> MLGTGPAAATTAATTSSNVSVLQQFASGLKSRNEETRAKAAKELQHYVTMELREMSQEESTRFYDQLNHHIFELVSSSDANERKGGILAIASLIGVEGGNATRIGRFANYLRNLLPSNDPVVMEMASKAIGRLAMAGDTFTAEYVEFEVKRALEWLGADRNEGRRHAAVLVLRELAISVPTFFFQQVQPFFDNIFVAVWDPKQAIREGAVAALRACLILTTQREPKEMQKPQWYRHTFEEAEKGFDETLAKEKGMNRDDRIHGALLILNELVRISSMEGERLREEMEEITQQQLVHDKYCKDLMGFGTKPRHITPFTSFQAVQPQQSNALVGLLGYSSHQGLMGFGTSPSPAKSTLVESRCCRDLMEEKFDQVCQWVLKCRNSKNSLIQMTILNLLPRLAAFRPSAFTDTQYLQDTMNHVLSCVKKEKERTAAFQALGLLSVAVRSEFKVYLPRVLDIIRAALPPKDFAHKRQKAMQVDATVFTCISMLARAMGPGIQQDIKELLEPMLAVGLSPALTAVLYDLSRQIPQLKKDIQDGLLKMLSLVLMHKPLRHPGMPKGLAHQLASPGLTTLPEASDVGSITLALRTLGSFEFEGHSLTQFVRHCADHFLNSEHKEIRMEAARTCSRLLTPSIHLISGHAHVVSQTAVQVVADVLSKLLVVGITDPDPDIRYCVLASLDERFDAHLAQAENLQALFVALNDQVFEIRELAICTVGRLSSMNPAFVMPFLRKMLIQILTELEHSGIGRIKEQSARMLGHLVSNAPRLIRPYMEPILKALILKLKDPDPDPNPGVINNVLATIGELAQVSGLEMRKWVDELFIIIMDMLQDSSLLAKRQVALWTLGQLVASTGYVVEPYRKYPTLLEVLLNFLKTEQNQGTRREAIRVLGLLGALDPYKHKVNIGMIDQSRDASAVSLSESKSS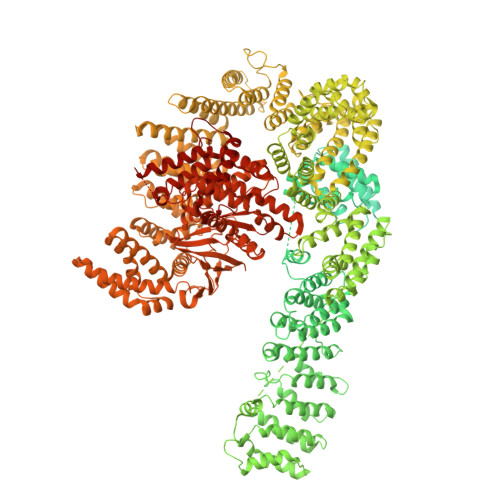QDSSDYSTSEMLVNMGNLPLDEFYPAVSMVALMRIFRDQSLSHHHTMVVQAITFIFKSLGLKCVQFLPQVMPTFLNVIRVCDGAIREFLFQQLGMLVSFVKSHIRPYMDEIVTLMREFWVMNTSIQSTIILLIEQIVVALGGEFKLYLPQLIPHMLRVFMHDNSPGRIVSIKLLAAIQLFGANLDDYLHLLLPPIVKLFDAPEAPLPSRKAALETVDRLTESLDFTDYASRIIHPIVRTLDQSPELRSTAMDTLSSLVFQLGKKYQIFIPMVNKVLVRHRINHQRYDVLICRIVKGYTLADEEEDPLIYQHRMLRSGQGDALASGPVETGPMKKLHVSTINLQKAWGAARRVSKDDWLEWLRRLSLELLKDSSSPSLRSCWALAQAYNPMARDLFNAAFVSCWSELNEDQQDELIRSIELALTSQDIAEVTQTLLNLAEFMEHSDKGPLPLRDDNGIVLLGERAAKCRAYAKALHYKELEFQKGPTPAILESLISINNKLQQPEAAAGVLEYAMKHFGELEIQATWYEKLHEWEDALVAYDKKMDTNKDDPELMLGRMRCLEALGEWGQLHQQCCEKWTLVNDETQAKMARMAAAAAWGLGQWDSMEEYTCMIPRDTHDGAFYRAVLALHQDLFSLAQQCIDKARDLLDAELTAMAGESYSRAYGAMVSCHMLSELEEVIQYKLVPERREIIRQIWWERLQGCQRIVEDWQKILMVRSLVVSPHEDMRTWLKYASLCGKSGRLALAHKTLVLLLGVDPSRQLDHPLPTVHPQVTYAYMKNMWKSARKIDAFQHMQHFVQTMQQQAQHAIATEDQQHKQELHKLMARCFLKLGEWQLNLQGINESTIPKVLQYYSAATEHDRSWYKAWHAWAVMNFEAVLHYKHQNQARDEKKKLRHASGANITNATTAATTAATATTTASTEGSNSESEAESTENSPTPSPLQKKVTEDLSKTLLMYTVPAVQGFFRSISLSRGNNLQDTLRVLTLWFDYGHWPDVNEALVEGVKAIQIDTWLQVIPQLIARIDTPRPLVGRLIHQLLTDIGRYHPQALIYPLTVASKSTTTARHNAANKILKNMCEHSNTLVQQAMMVSEELIRVAILWHEMWHEGLEEASRLYFGERNVKGMFEVLEPLHAMMERGPQTLKETSFNQAYGRDLMEAQEWCRKYMKSGNVKDLTQAWDLYYHVFRRISKQLPQLTSLELQYVSPKLLMCRDLELAVPGTYDPNQPIIRIQSIAPSLQVITSKQRPRKLTLMGSNGHEFVFLLKGHEDLRQDERVMQLFGLVNTLLANDPTSLRKNLSIQRYAVIPLSTNSGLIGWVPHCDTLHALIRDYREKKKILLNIEHRIMLRMAPDYDHLTLMQKVEVFEHAVNNTAGDDLAKLLWLKSPSSEVWFDRRTNYTRSLAVMSMVGYILGLGDRHPSNLMLDRLSGKILHIDFGDCFEVAMTREKFPEKIPFRLTRMLTNAMEVTGLDGNYRITCHTVMEVLREHKDSVMAVLEAFVYDPLLNWRLMDTNTKGNKRSRTRTDSYSAGQSVEILDGVELGEPAHKKTGTTVPESIHSFIGDGLVKPEALNKKAIQIINRVRDKLTGRDFSHDDTLDVPTQVELLIKQATSHENLCQCYIGWCPFW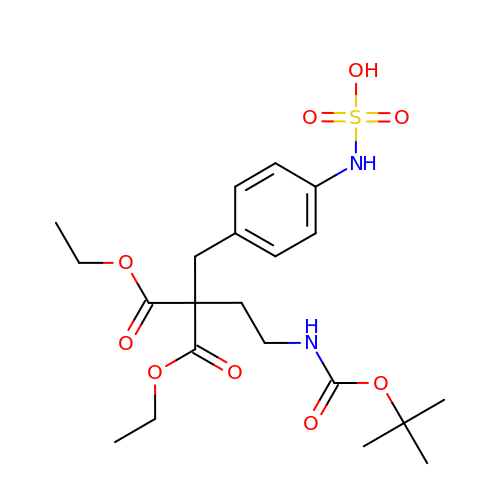(4-{4-[(TERT-BUTOXYCARBONYL)AMINO]-2,2-BIS(ETHOXYCARBONYL)BUTYL}PHENYL)SULFAMIC ACID | C21 H32 N2 O9 S | VHLMZWXTBDMYOE-UHFFFAOYSA-N>RKPRGRPKKX[4x]

High mobility group A proteins (HMGA, formerly called HMG-I/Y) are intrinsically disordered non-histone chromosomal proteins characterized by containing three DNA-binding domains, called AT-hooks, which preferentially bind to the minor groove of short stretches of AT-rich DNA. By binding to differently spaced AT-rich DNA regions and/or direct interaction with several transcription factors, HMGAs regulate the expression of numerous genes. The HMGA1 protein contains three AT-hooks. All of them are formed by a conserved core sequence, Pro-Arg-Gly-Arg-Pro, flanqued by positively charged amino acids.

In our studies we have used a peptide with nine amino acids identical to those found in DBD3 and similar to those found in DBD2. As shown in the Methods section our crystals contain four complexes which are very similar. The geometry of the duplex and the central sequence of the AT-hook (PRGRP) are practically identical in the four complexes. On the other hand the external AT-hook terminal amino acids vary in each of the four complexes present in our crystal. The DNA duplex has a clear bend, localized in the region of base pairs 5 and 6. It determines an angle of 24° between the lower five bases and the upper seven bases of the duplex. The minor groove in one of them is occupied by the AT-hook, whereas the other region shows a clear spine of hydration, typical for the AATT sequence. The minor groove is wide in the region occupied by the AT-hook, with phosphate-phosphate distances in the range 12–13 Å. A clear hydrogen bond of the main chain NH group of Arg-38 is formed with one thymine oxygen. However the main lesson of our work is that the AT-hook can bind to a strongly distorted DNA molecule, whereas most models of interaction assume that the B form of DNA remains practically unchanged upon binding.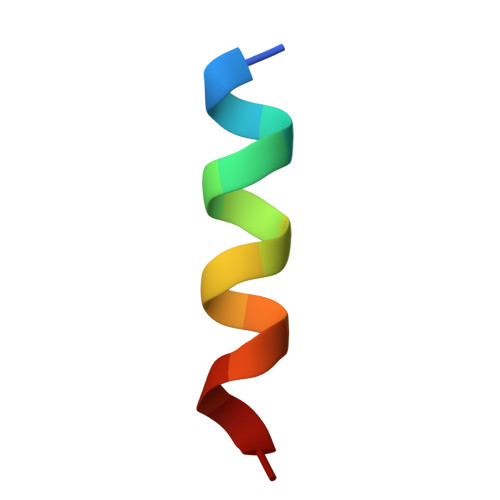> SLMRVQAHIRKRMVA> SGFSAEKYEQIQFGMTFDEVWEIGGGEAACDTGGVIGDSILCFTESGDYAPYGGFSFTDEGELWSKRNEYLYKAKTPSVKLSHYNRTALGMTEAQLWAAVPKDSCVSQGESYPNWPAKTGFEEKYYC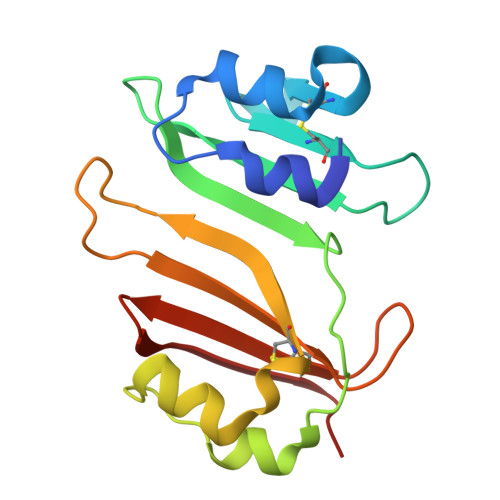AAATGLFPPSASFHLTDGVLTYRYQRSLT>[2x]GNADEXYKEL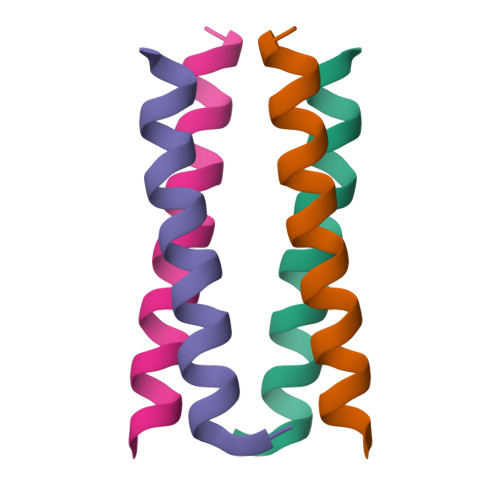EDXQERLRKXRKKLRS>[2x]MTIN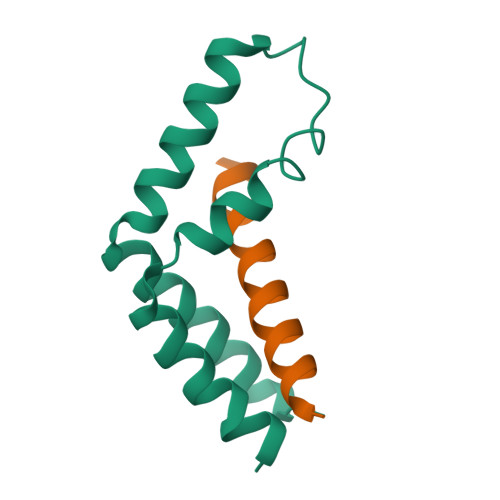KETGTDPDPGYKPTLRSQDKAALKELLHTRLVECGWHKDIKEMIRNIIMERGVDNINRDQLAAQIVPQARALVPEVVKNEMMLRVHAALDK;>SGSLDEAANYLYQSLLDDAVVGIFNETHHLRKSGNLAALDGV[2x]> LKESPSGYLRSGEGDTGCGELVWVGEPLTLRTAETITGKYGVWMRDPKPTYPYTQETTWRIDTVGTDVRQVFEYDLISQFMQGYP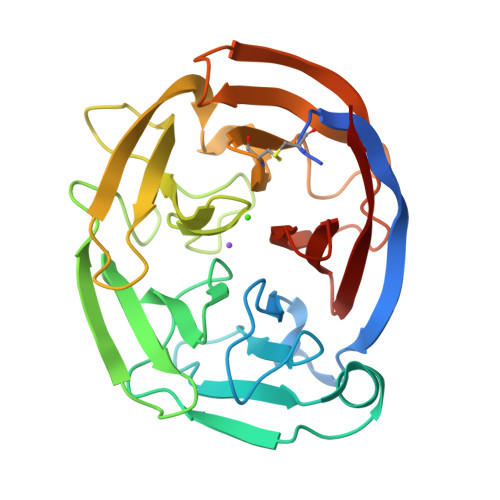SKVHILPRPLESTGAVVYLGSLYFQGAESRTVIRYELNTETVKAEKEIPGAGYHGQFPYSWGGYTDIDLAVDEAGLWVIYSTDEAKGAIVLSKLNPENLELEQTWETNIRKQSVANAFIICGTLYTVSSYTSADATVNFAYDTGTGISKTLTIPFKNRYKYSSMIDYNPLEKKLFAWDNLNMVTYDIKLSKM Ribonuclease P (RNase P) is the essential endonuclease that catalyzes the 5’-end maturation of tRNAs. More recently, a bacterial protein-only RNase P, associated with a single polypeptide as small as ~23 kDa, was discovered in the hyperthermophilic bacterium Aquifex aeolicus that lost the genes for the RNA and protein subunits (rnpB and rnpA) of the classical and ancient bacterial RNase P. This prokaryotic type of minimal RNase P system was named HARP (for: Homolog of Aquifex RNase P) and identified in 5 other of the 36 bacterial phyla beyond Aquificae. HARPs belong to the PIN domain-like superfamily of metallonucleases. Homologs of Aquifex RNase P (HARPs) are also expressed in some other bacteria and many archaea, where they coexist with RNA-based RNase P and do not represent the main RNase P activity.

Here, we present the homo-dodecameric structure of the HARP from the γ-bacterium Halorhodospira halophila SL1 (Hhal2243) solved by cryo-electron microscopy (EM) at 3.37 Å resolution. Hhal2243 assembles into a dodecamer in a left-handed screw-like manner, with each molecule being rotated by approximately 58°, except for the interface between dimers 1/1* and 6/6*. Upon completion of the single screw turn, the first and last dimers (1/1* and 6/6*) encounter each other at a slightly larger angle of 70° (top view, left) and laterally displaced (side view, right); they cannot form the same inter-dimer contacts as dimers can form within the screw turn; the steric clash between dimers 1/1* and 6/6* terminates oligomerization. Hhal2243 consists of a PIN-like metallonuclease domain into which two helices are inserted that we termed the ‘spike-helix’ (SH) domain. The PIN-like domain is formed by six α-helices (α1–α4, α7, and α8) and four β-strands (β1–β4) that fold into an α/β/α domain with a central, four-stranded parallel β-sheet. Two Hhal2243 monomers align head-to-head with their SH domains consisting of helices α5 and α6 to form a dimer, while two SH domains form a four-helix bundle resulting in six spikes that protrude from the dodecameric assembly. The dimer interface covers a buried surface area of 1300 Å2 and is mainly of hydrophobic nature with two clamping salt bridges formed by R141 and E91 from either monomer, respectively. The covered interface between neighboring dimers extends over 900 Å2 and involves the long α4–α5 loop of one monomer and the α7–α8 loop as well as helix α8 of the respective other monomer. Application of this method to Hhal2243 revealed a stable dodecameric assembly of 295 kDa that included 98% of all molecules in the sample. Our Hhal2243 structure supports the prediction that these residues constitute the active site of the protein, including an almost perfect superposition with three of the four active site aspartates of AtPRORP1 (D399, D475, and D493; Howard et al., 2012).

>GSHMASRRFVLDTSVFTNPDVYLRFDEEPMQAISVFLGLARRADAEFYMPGPVYQELCNLRSMDLIGAEFETEVYIRSPRRFSMTIPSEVLYEFIEEVRTRIQRGLRIAEEHARQAGQAESLPPELITQLRERYREAMRRGILDSREDIDVVLLAYELDATLVSADEGMRKFAERIGIKLVNPRYLRGVMQNLAGDDPGHAPPCGPDQPAG[12x]>[6x]MVLSHAVSESDVSVHSTFASRYVRTSLPRFKMPENSIPKEAA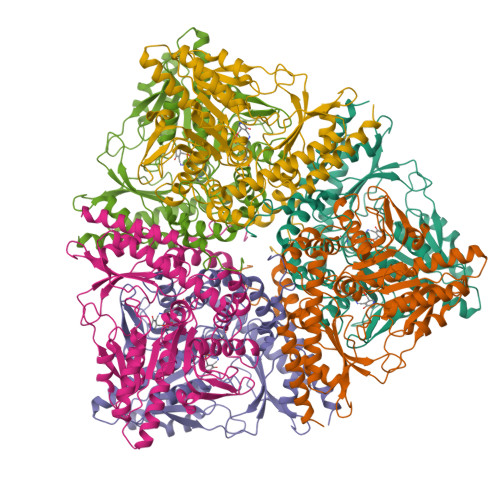YQIINDELMLDGNPRLNLASFVTTWMEPECDKLIMSSINKNYVDMDEYPVTTELQNRCVNMIAHLFNAPLEEAETAVGVGTVGSSEAIMLAGLAFKRKWQNKRKAEGKPVDKPNIVTGANVQVCWEKFARYFEVELKEVKLSEGYYVMDPQQAVDMVDENTICVAAILGSTLNGEFEDVKLLNDLLVEKNKETGWDTPIHVDAASGGFIAPFLYPELEWDFRLPLVKSINVSGHKYGLVYAGIGWVIWRNKEDLPEELIFHINYLGADQPTFTLNFSKGSSQVIAQYYQLIRLGHEGYRNVMENCRENMIVLREGLEKTERFNIVSKDEGVPLVAFSLKDSSCHTEFEISDMLRRYGWIVPAYTMPPNAQHITVLRVVIREDFSRTLAERLVIDIEKVMRELDELPSRVIHKISLGQEKSESNSDNLMVTVKKSDIDKQRDIITGWKKFVADRKKTSGIC>STLDFYAQGQGDRLIDPARFPAEIKAFLEGERVLLDSVAEHVELLVEVGSMHGQHLGWAIARGKHYIGVDPVPRYIEQGRRTLREQGLPAERFRFIEGGAEELHQLLPRHALAVPPSRCLLFFPFNSFGNMRDPERVLESLSMTGLPFLISSYATTERATQARAAYYAQCQYEWLESACDERGVRFRAPEGFDAMAYHVEYLEPRMRRYGLEVRPIPFADVGVAWCAGPMFEPWRP[2x]

AZE synthases catalyse the intramolecular 4-exo-tet cyclisation of S-adenosylmethionine (SAM), yielding a highly strained heterocycle. More recently, AZE synthases have been discovered in bacteria, namely AzeJ and VioH, which are involved in the biosynthesis of azetidomonamides and vioprolides, respectively. Interestingly, they show sequence similarity to the class I methyltransferases (MT1). Each subunit adopts a classic Rossmann fold, consisting of a 7-stranded β-sheet (β3↑, β2↑, β1↑, β4↑, β5↑, β10↓, β9↑) surrounded by helices α4-6, α8-9 and α11, a topology that is typical for MT1 enzymes.

To gain a better understanding of the intramolecular cyclisation reaction of SAM to MTA and AZE, we determined the high-resolution structures of AzeJ and VioH. In contrast, we were able to obtain crystals in the presence of SAM or S-adenosyl-L-homocysteine (SAH), which diffracted up to 1.95 Å. Our analyses revealed that AzeJ forms a homodimer, whilst VioH is monomeric. Although the sequence identity between AzeJ and VioH is only 28%, their monomers share a remarkable structural similarity (backbone root mean square deviation (rmsd) = 1.8 Å, 72% Cα-atoms). Nevertheless, the catalysis in AzeJ and VioH would follow the same mechanistic principles, given their structural similarity. Indeed, a DFT cluster model of VioH, in which water molecules are bound near the sulfonium, reveals a high reaction barrier of ca. 23 kcal mol−1 in agreement with its low activity towards SAM. Intriguingly, co-expression of pxaA with azeJ led to the production of 3, which is in contrast to the experiment with pxaA and vioH and consistent with the in vitro observation that VioH alone had minimal catalytic activity.N6-{[(6-aminopyridin-3-yl)methoxy]carbonyl}-L-lysine | C13 H20 N4 O4 | 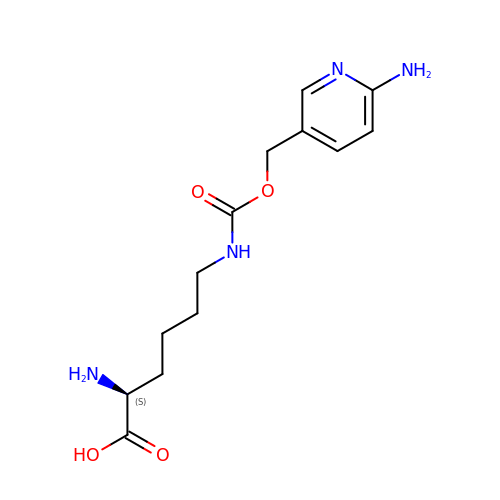BRYLMTIKKYDVII-JTQLQIEISA-N>[2x]MEAFEISDFKEHAKKKSMWAGALNKVTISGLMGVFTEDEDLMALPIHRDHCPALLKIFDEIIVNATDHERACHNKTKKVTYIKISFDKGVFSCENDGPGIPIAKHEQASLIAKRDVYVPEVASCHFLAGTNINKAKDCIKGGTNGVGLKLAMVHSQWAILTTADGAQKYVQHINQRLDIIEPPTITPSREMFTRIELMPVYQELGYAEPLSETEQADLSAWIYLRACQCAAYVGKGTTIYYNDKPCRTGSVMALAKMYTLLSAPNSTIHTATIKADAKPYSLHPLQVAAVVSPKFKKFEHVSVINGVNCVKGEHVTFLKKTINEMVVKKFQQTIKDKNRKTTLRDSCSNIFIVIVGSIPGIEWTGQRKDELSIAENVFKTHYSIPSSFLTSMTKSIVDILLQSISKKDNHKQVDVDKYTRARNAGGKRAQDCMLL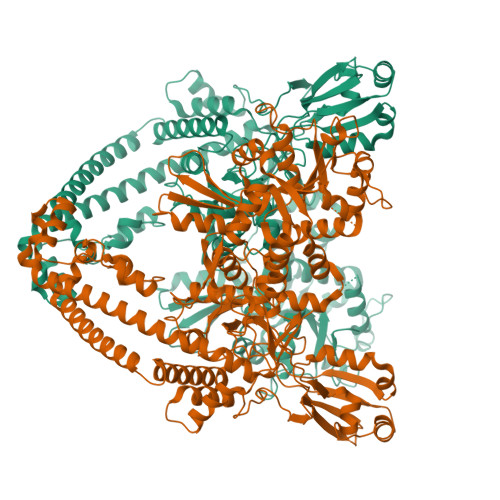AAEGDSALSLLRTGLTLGKSNPSGPSFDFCGMISLGGVIMNACKKVTNITTDSGETIMVRNEQLTNNKVLQGIVQVLGLDFNCHYKTQEERAKLRYGCIVACVDQDLDGCGKILGLLLAYFHLFWPQLIIHGFVKRLLTPLIRVYEKGKTMPVEFYYEQEFDAWAKKQTSLANHTVKYYKGLAAHDTHEVKSMFKHFDNMVYTFTLDDSAKELFHIYFGGESELRKRELCTGVVPLTETQTQSIHSVRRIPCSLHLQVDTKAYKLDAIERQIPNFLDGMTRARRKILAGGVKCFASNNRERKVFQFGGYVADHMFYHHGDMSLNTSIIKAAQYYPGSSHLYPVFIGIGSFGSRHLGGKDAGSPRYISVQLASEFIKTMFPAEDSWLLPYVFEDGQRAEPEYYVPVLPLAIMEYGANPSEGWKYTTWARQLEDILALVRAYVDKDNPKHELLHYAIKHKITILPLRPSNYNFKGHLKRFGQYYYSYGTYVISEQRNIITITELPLRVPTVAYIESIKKSSNRMTFIEEIIDYSSSETIEILVKLKPNSLNRIVEEFKETEEQDSIENFLRLRNCLHSHLNFVKPKGGIIEFNTYYEILYAWLPYRRELYQKRLMREHAVLKLRIIMETAIVRYINESAELNLSHYEDEKEASRILSEHGFPPLNHTLIISPEFASIEELNQKALQGCYTYILSLQARELLIAAKTRRVEKIKKMQARLDKVEQLLQESPFPGASVWLEEIDAVEKAIIKGRNTQWKFH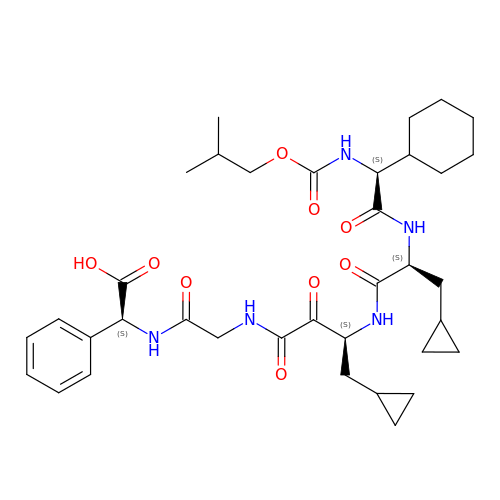[(N-{3-[(N-{CYCLOHEXYL[(ISOBUTOXYCARBONYL)AMINO]ACETYL}-3-CYCLOPROPYLALANYL)AMINO]-4-CYCLOPROPYL-2-OXOBUTANOYL}GLYCYL)AMINO](PHENYL)ACETIC ACID | C36 H51 N5 O9 | VZZMJPCOMQVXJP-ZHTHUIBPSA-N> MKFGLFFLNFMNSKRSSDQVIEEMLDTAHYVDQLKFDTLAVYENHFSNNGVVGAPLTVAGFLLGMTKNAKVASLNHVITTHHPVRVAEEACLLDQMSEGRFAFGFSDCEKSADMRFFNRPTDSQFQLFSECHKIINDAFTTGYCHPNNDFYSFPKISVNPHAFTEGGPAQFVNATSKEVVEWAAKLGLPLVFRWDDSNAQRKEYAGLYHEVAQAHGVDVSQVRHKLTL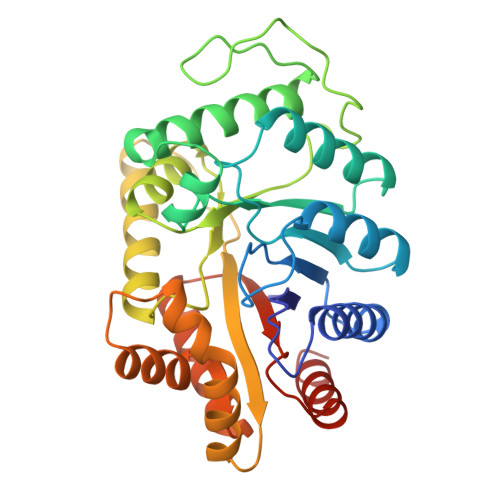LVNQNVDGEAARAEARVYLEEFVRESYSNTDFEQKMGELLSENAIGTYEESTQAARVAIECCGAADLLMSFESMEDKAQQRAVIDVVNANIVKYHS>[2x]MSEPEVPFKVVAQFPYKSDYEDDLNFEKDQEIIVTSVEDAEWYFGEY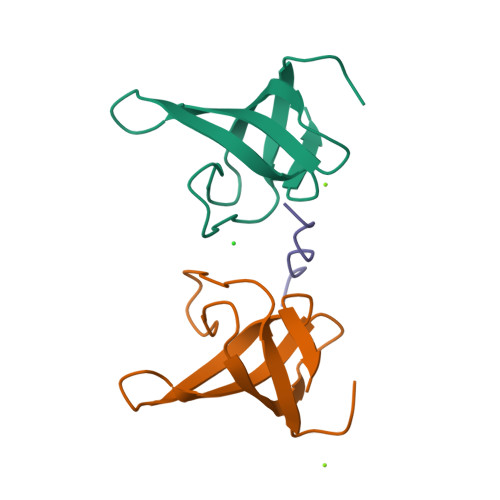QDSNGDVIEGIFPKSFVAVQG;> RGPAPPPPPHR> SESSESKASSGLPIDLRGKRAFIAGIADDNGYGWAVAKSLAAAGAEILVGTWVPALNIFETSLRRGKFDQSRVLPDGSLMEIKKVYPLDAVFDNPEDVPEDVKANKRYAGSSNWTVQEAAECVRQDFGSIDILVHSLANGPEVSKPLLETSRKGYLAAISASSYSFVSLLSHFLP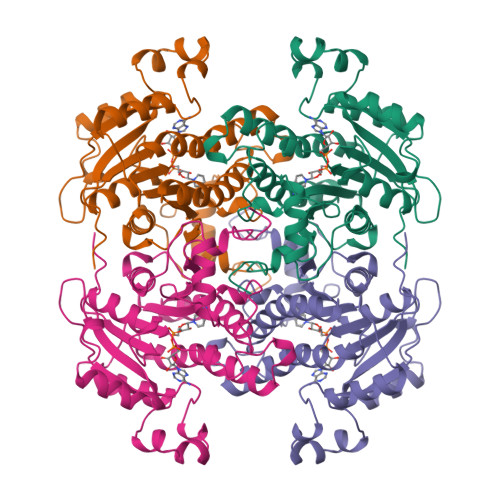IMNPGGASISLTYIASERIIPGYGGGMSSAKAALESDTRVLAFEAGRKQNIRVNTISAGPLGSRAAKAIGFIDTMIEYSYNNAPIQKTLTADEVGNAAAFLVSPLASAITGATIYVDNGLNSMGVALDSPVFKDLDK>[4x]GSPRTVEEIFKDYSARRAALLRALTKDVDDFYSQCDPEKENLCLYGHPNESWEVNLPAEEVPPELPEPALGINFAR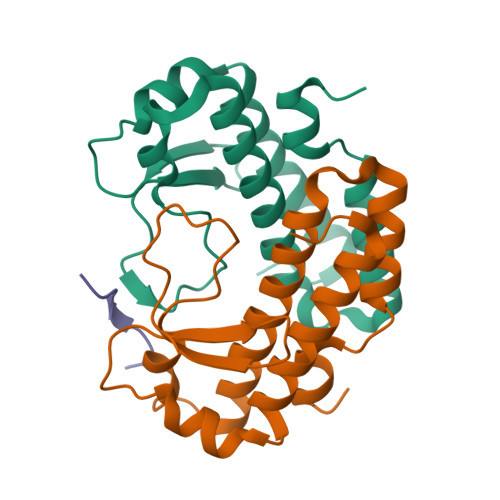DGMQRKDWLSLVAVHSDCWLLSVSFYFGARLNRNERKRLFSLINDLPTLFDVVTGRKAM;>ETVTPKRMRTTQRKRSAT[2x]>[2x]HNKVRTCWNEGRPALAGWLQLPGTLHAEALARLDYDAVVIDMQHSPIDFGQVAPMLIAIELGGAEPFVRTQVNDPSDIMKLLDAGAYGIIAPMVNTRAEAQTLASALHYSPRGLRAFGPRRPSLRYGSGYLAQASETVVGLAMIETREALANIDEILSVDGIDGVFIGPTDLALDLGHAPLVDTEEAEVVSAIAHVRERAHAAGKRVGIFCGSGGFARVKLAEGFDFVTAAPDLAMLSAAARQVIADARAL

Here structural analysis of hydroxyketoacid aldolase from Sphingomonas wittichii RW1 (SwHKA) revealed a dynamic movement of the metal cofactor between two coordination spheres without protein scaffold rearrangements. Holo‐SwHKA forms a trimer of homodimers, in which each monomer adopts an (α/β)8 triosephosphate isomerase (TIM) barrel fold. In total, holo‐SwHKA contains six equivalent active sites; each of which is formed from amino acids from two different domain‐swapped dimers. The transition from M2+ R to M2+ A,S is induced by bidentate substrate binding and occurs without a concomitant rearrangement of the protein scaffold.

To investigate a potential structural role for the metal cofactor in the M2+ R configuration through interactions with residue S116′, two different variants were designed at this position. Notably, mutagenesis at position S116 reduced the expression yield of soluble protein by more than 10‐fold down to ≈3 mg L−1 of expression medium. Identical orientations of the alanine/serine residues were observed, and the protein fold was unaffected by the mutation (rmsd=0.115 Å between 230 Cα atoms). Surprisingly, no significant difference was observed between the wild‐type and S116 A variants of SwHKA upon holoenzyme formation with MgCl2, as the thermal stability of all variants increased by ≈7 °C. This suggests that the thermal unfolding of SwHKA is not initiated by the dissociation of the trimer of the domain‐swapped dimers. For the S116A mutant, a lower apparent K d (i.e. higher affinity) toward M2+ A,S was observed with Mg2+, while the affinity remained mostly unaffected when Mn2+ was used. These data suggest that elimination of M2+ R could remove the competition between the two binding modes, and thereby increase its affinity toward the M2+ A,S configuration.> AAQTNAPWGLARISSTSPGTSTYYYDESAGQGSCVYVIDTGIEASHPEFEGRAQMVKTYYYSSRDGNGHGTHCAGTVGSRTYGVAKKTQLFGVKVLDDNGSGQYSTIIAGMDFVASDKNNRN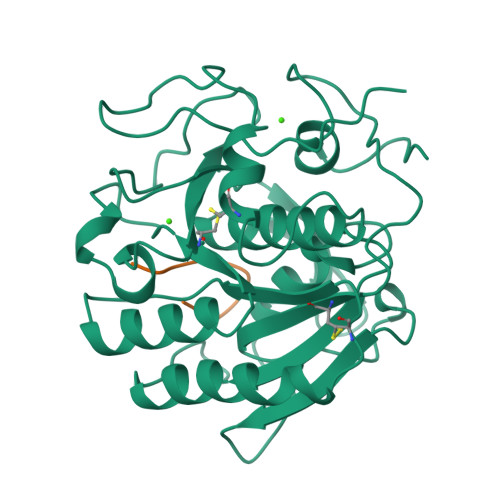CPKGVVASLSLGGGYSSSVNSAAARLQSSGVMVAVAAGNNNADARNYSPASEPSVCTVGASDRYDRRSSFSNYGSVLDIFGPGTSILSTWIGGSTRSISGTSMATPHVAGLAAYLMTLGKTTAASACRYIADTANKGDLSNIPFGTVNLLAYNNYQA;> VAQGGAAGLA> GAMGSGLAKYLPGATNLLSKSGEVSLGSLVGKTVFLYFSASWCPPCRGFTPVLAEFYEKHHVAKNFEVVLISWDENESDFHDYYGKMPWLALPFDQRSTVSEL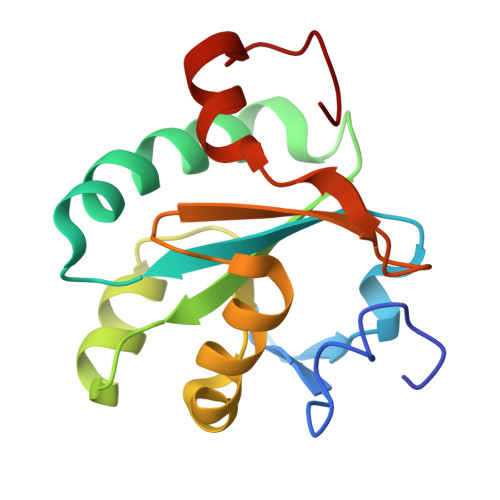GKTFGVESIPTLITINADTGAIIGTQARTRVIEDPDGANFPW>[3x]LLPVKYCKMRIFSGSTAAAPEEEPFEVWLEQATEIAKEWPIPEAEKKRWVAE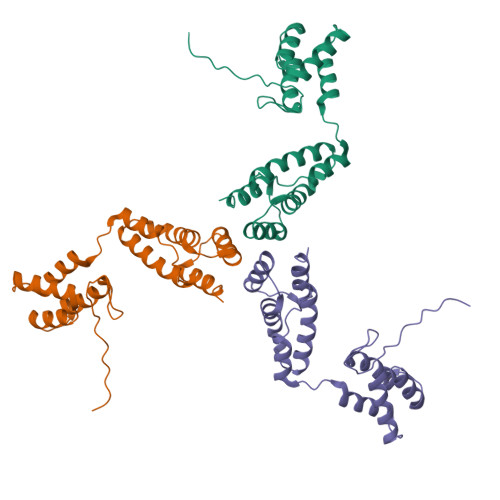SLRGPALDLMHIVQADNPSISVGECLEAFKQVFGSTESRRTSQVKYLRTYQQEGEKISAYVLRLETLLRRAVEKRAIPRNIADQVRLEQVMAGANLGNVLWCRLQELKDQGPLPTFLQLMKVIREEEE> MNIQKIQKLIENGTTLLLSIEDCVGSNYDLALDLHKRNSDEIPEDVIINNNAKNYETMRELIVKITADGEGLNKGMATVDVKKLSEMVSLFEQKYLETELARHDIFGELISRHLRIKPKQRSEVEIEHALREYLDELNKKSCINKLSDDEFERINKEYVATNATPDNYVIYKESKNSELCLIIYDWKISVDARTETKTMEKYYKNIWKSFKDIKVNGKPFLEDHPVFVSIVILKPIAGMPIT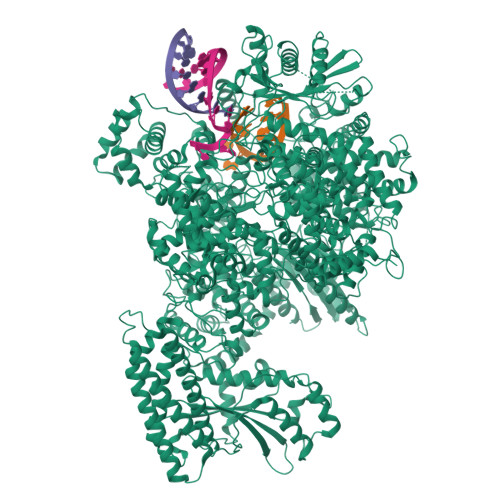VTSSRVLEKFEDSPSALHGERIKHARNAKLLNISHVGQIVGTTPTVVRNYYANTQKIKSEVRGILGDDFGSKDVFFSHWTSKYKERNPTEIAYSEDIERIIDSLVTDEITKEEIIHFLFGNFCFHIETMNDQHIADKFKGYQSSCINLKIEPKVDLADLKDHLIQKQQIWESLYGKHLEKIMLRIREKKKKEKEIPDITTAFNQNAAEYEEKYPNCFTNDLSETKTNFSMTWSPSFEKIELSSEVDYNNAIINKFRESFKSSSRVIYNSPYSSINNQTNKARDITNLVRLCLTELSCDTTKMEKQELEDEIDINTGSIKVERTKKSKEWNKQGSCLTRNKNEFCMKETGRENKTIYFKGLAVMNIGMSSKKRILKKEEIKERISKGLEYDTSERQADPNDDYSSIDMSSLTHMKKLIRHDNEDSLSWCERIKDSLFVLHNGDIREEGKITSVYNNYAKNPECLYIQDSVLKTELETCKKINKLCNDLAIYHYSEDMMQFSKGLMVADRYMTKESFKILTTANTSMMLLAFKGDGMNTGGSGVPYIALHIVDEDMSDQFNICYTKEIYSYFRNGSNYIYIMRPQRLNQVRLLSLFKTPSKVPVCFAQFSKKANEMEKWLKNKDIEKVNVFSMTMTVKQILINIVFSSVMIGTVTKLSRMGIFDFMRYAGFLPLSDYSNIKEYIRDKFDPDITNVADIYFVNGIKKLLFRMEDLNLSTNAKPVVVDHENDIIGGITDLNIKCPITGSTLLTLEDLYNNVYLAIYMMPKSLHNHVHNLTSLLNVPAEWELKFRKELGFNIFEDIYPKKAMFDDKDLFSINGALNVKALSDYYLGNIENVGLMRSEIENKEDFLSPCYKISTLKSSKKCSQSNIISTDEIIECLQNAKIQDIENWKGNNLAIIKGLIRTYNEEKNRLVEFFEDNCVNSLYLVEKLKEIINSGSITVGKSVTSKFIRNNHPLTVETYLKTKLYYRNNVTVLKSKKVSEELYDLVKQFHNMMEIDLDSVMNLGKGTEGKKHTFLQMLEFVMSKAKNVTGSVDFLVSVFEKMQRTKTDREIYLMSMKVKMMLYFIEHTFKHVAQSDPSEAISISGDNKIRALSTLSLDTITSYNDILNKNSKKSRLAFLSADQSKWSASDLTYKYVLAIILNPILTTGEASLMIECILMYVKLKKVCIPTDIFLNLRKAQGTFGQNETAIGLLTKGLTTNTYPVSMNWLQGNLNYLSSVYHSCAMKAYHKTLECYKDCDFQTRWIVHSDDNATSLIASGEVDKMLTDFSSSSLPEMLFRSIEAHFKSFCITLNPKKSYASSSEVEFISERIVNGAIIPLYCRHLANCCTESSHISYFDDLMSLSIHVTMLLRKGCPNEVIPFAYGAVQVQALSIYSMLPGEVNDSIRIFKKLGVSLKSNEIPTNMGGWLTSPIEPLSILGPSSNDQIIYYNVIRDFLNKKSLEEVKDSVSSSSYLQMRFRELKGKYEKGTLEEKDKKMIFLINLFEKASVSEDSDVLTIGMKFQTMLTQIIKLPNFINENALNKMSSYKDFSKLYPNLKKNEDLYKSTKNLKIDEDAILEEDELYEKIASSLEMESVHDIMIKNPETILIAPLNDRDFLLSQLFMYTSPSKRNQLSNQSTEKLALDRVLRSKARTFVDISSTVKMTYEENMEKKILEMLKFDLDSYCSFKTCVNLVIKDVNFSMLIPILDSAYPCESRKRDNYNFRWFQTEKWIPVVEGSPGLVVMHAVYGSNYIENLGLKNIPLTDDSINVLTSTFGTGLIMEDVKSLVKGKDSFETEAFSNSNECQRLVKACNYMIAAQNRLLAINTCFTRKSFPFYSKFNLGRGFISNTLALLSTIYSKEES> ILPQPDVRVNQVGYLPEGKKVATVVCNSTQPVKWQLKNAAGVVVLEGYTEPKGLDKDSQDYVHWLDF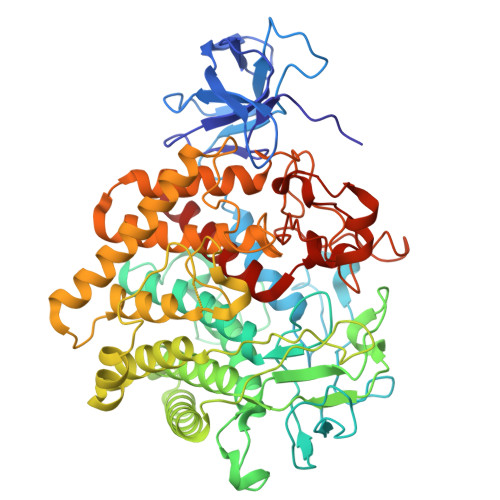SDFATEGIGYYFELPTVNSPTNYSHPFDIRKDIYTQMKYDALAFFYHKRSGIPIEMPYAGGEQWTRPAGHIGIEPNKGDTNVPTWPQDDEYAGIPQKNYTKDVTGGWYDAGDHGKYVVNGGIAVWTLMNMYERAKIRGLDNWGPYRDGGMNIPEQNNGYPDILDEARWEIEFFKKMQVTEKEDPSIAGMVHHKIHDFRWTALGMLPHEDPQPRYLRPVSTAATLNFAATLAQSARLWKDYDPTFAADCLEKAEIAWQAALKHPDIYAEYTPGSGGPGGGPYNDDYVGDEFYWAACELYVTTGKDEYKNYLMNSPHYLEMPAKMGENGGANGEDNGLWGCFTWGTTQGLGTITLALVENGLPATDIQKARNNIAKAADRWLENIEEQGYRLPIKQAEDERGGYPWGSNSFILNQMIVMGYAYDFTGDSKYLDGMFDGISYLLGRNAMDQSYVTGYGERPLQNPHDRFWTPQTSKRFPAPPPGIISGGPNSRFEDPTINAAVKKDTPPQKCFIDHTDSWSTNEITVNWNAPFAWVTAYLDQYTD>MKDGMRVGERFTHDFVVPPHKTVRHLYPESPEFAEFPEVFATGFMVGLMEWACVRAMAPYLEPGEGSLGTAICVTHTAATPPGLTVTVTAELRSVEGRRLSWRVSAHDGVDEIGSGTHERAVIHL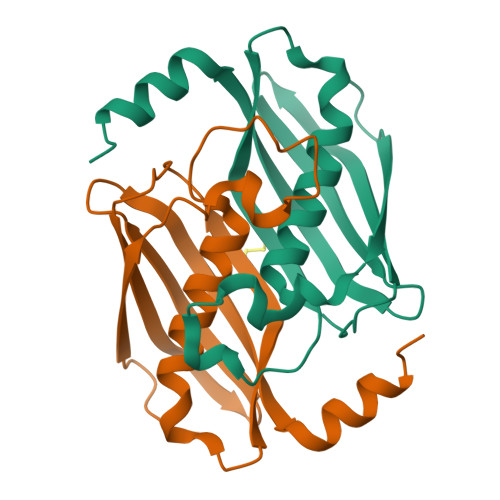EKFNAKVRQKTPAG[8x]> NSWGSQMDLTDPLCIEDDTENCKQTMSPNELGLTSAQDDGPLGQEKPNYFLNFRSMNVDIFTVSHTKVDNLFGRAWFFMEHTFTNEGQWRVPLEFPKQGHGSLSLLFAYFTGELNIHVLFLSERGFLRVAHTYDTSNDRVNFLSSNGVITVPAGEQMTLSAPYYSNKPLRTVRDNNSLGYLMCKPFLTGTSTGKIEV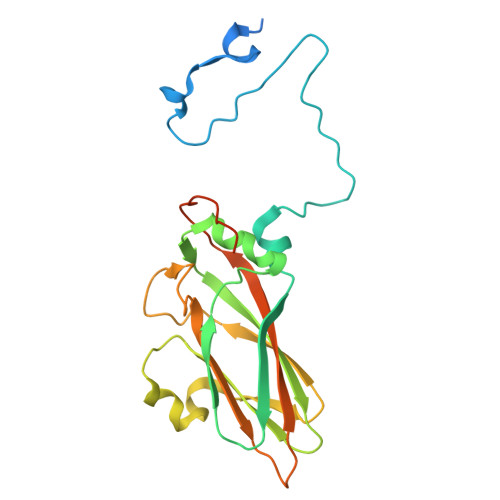YLSLRCPNFFFPLPAPKVTSSRALRGDMANLTNQSPY>MSGMILDELSWRGLIAQSTDLDTLAAEAQRGPMTVYAGFDPTAPSLHAGHLVPLLTLRRFQRAGHRPIVLAGGATGMIGDPRDVGERSLNEADTVAEWTERIRGQLERFVDFDDSPMGAIVENNLEWTGSLSAIEFLRDIGKHFSVNVMLARDTIRRRLAGEGISYTEFSYLLLQANDYVELHRRHGCTLQIGGADQWGNIIAGVRLVRQKLGATVHALTVPLVTAADGTKFGKSTGGGSLWLDPQMTSPYAWYQYFVNTADADVIRYLRWFTFLSADELAELEQATAQRPQQRAAQRRLASELTVLVHGEAATAA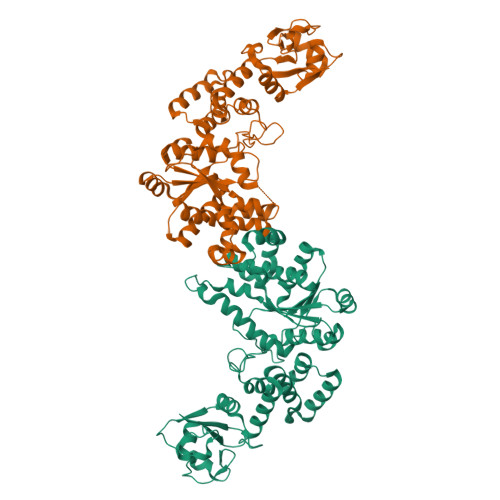VEHASRALFGRGELARLDEATLAAALRETTVAELKPGSPDGIVDLLVASGLSASKGAARRTIHEGGVSVNNIRVDNEEWVPQSSDFLHGRWLVLRRGKRSIAGVERIGLEHHHHHH[4x]> AEPSKAGQSAIENFQPVTADDLAGKNPANWPILRGNYQGWGYSPLDQINKDNVGDLQLVWSRTMEPGSNEGAAIAYNGVIFLGNTNDVIQAIDGKTGSLIWEYRRKLPSASK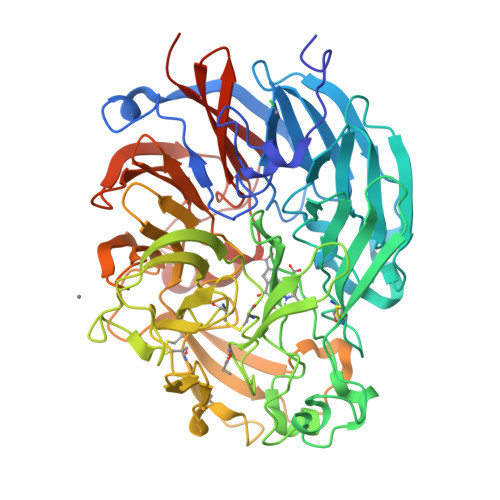FINSLGAAKRSIALFGDKVYFVSWDNFVVALDAKTGKLAWETNRGQGVEEGVANSSGPIVVDGVVIAGSTCQFSGFGCYVTGTDAESGEELWRNTFIPRPGEEGDDTWGGAPYENRWMTGAWGQITYDPELDLVYYGSTGAGPASEVQRGTEGGTLAGTNTRFAVKPKTGEVVWKHQTLPRDNWDSECTFEMMVVSTSVNPDAKADGMMSVGANVPRGETRKVLTGVPCKTGVAWQFDAKTGDYFWSKATVEQNSIASIDDTGLVTVNEDMILKEPGKTYNYCPTFLGGRDWPSAGYLPKSNLYVIPLSNACYDVMARTTEATPADVYNTDATLVLAPGKTNMGRVDAIDLATGETKWSYETRAALYDPVLTTGGDLVFVGGIDRDFRALDAESGKEVWSTRLPGAVSGYTTSYSIDGRQYVAVVSGGSLGGPTFGPTTPDVDSASGANGIYVFALPEKK>[2x]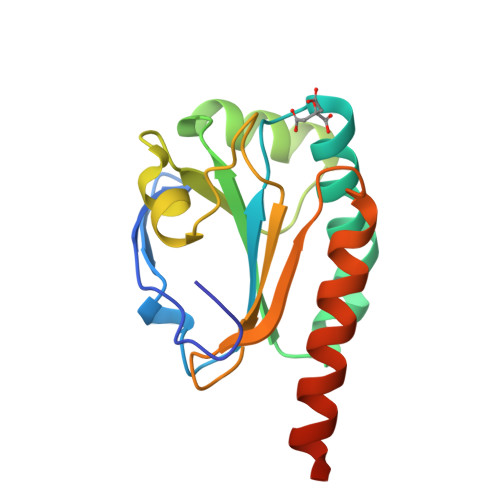MVKVGDKAPLFEGIADNGEKISLSDYIGKHNIVLYFYPKDDTPGSTREASAFRDNWDLLKDYDVVVIGVSSDDINSHKRFKEKYKLPFILVSDPDKKIRELYGAKGFILPARITFVIDKKGIIRHIYNSQMNPANHVNEALKALKQIKEEEISLEHHHHHH> MAEEWYFGKITRRESERLLLNPENPRGTFLVRESETTKGA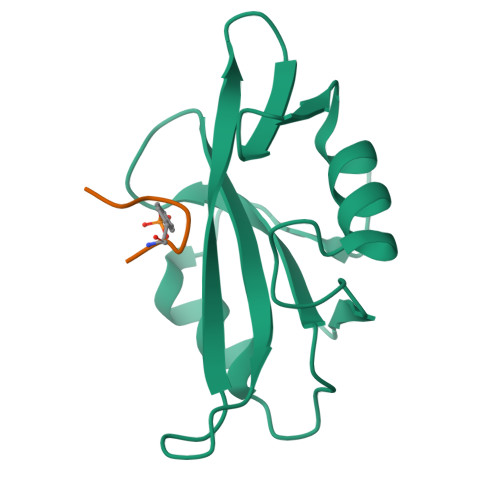YCLSVSDFDNAKGLNVKHYKIRKLDSGGFYIWSRTQFSSLQQLVAYYSKHADGLCHRLTNVCPT;> SYVNVQN> GASPSAQELKEQGNRLFVGRKYPEAAACYGRAITRNPLVAVYYTNRALCYLKMQQHEQALADCRRALELDGQSVKAHFFLGQCQLEMESYDEAIANLQRAYSLAKEQRLNFGDDIPSALRIA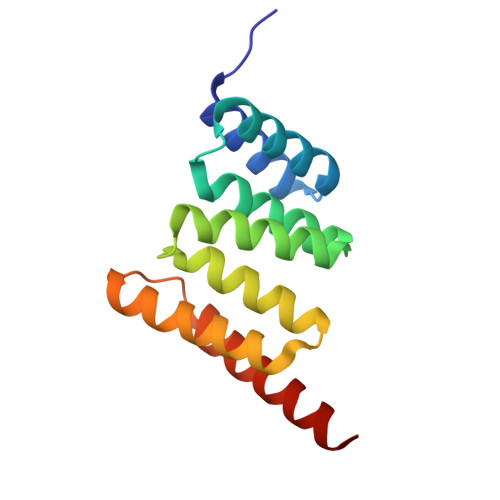KKKRWNSIEERR> HHHHHHMNTEKLETLLGFYKQYKALSEYIDKKYKLSLNDLAVLDLTMKHCKDEKVLMQSFLKTAMDELDLSRTKLLVSIRRLIE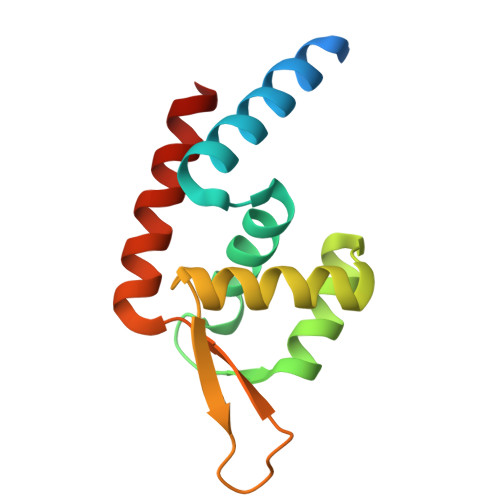KERLSKVRSSKDERKIYIYLNNDDISKFNALFEDVEQFLNI> MSLGAKPFGEKKF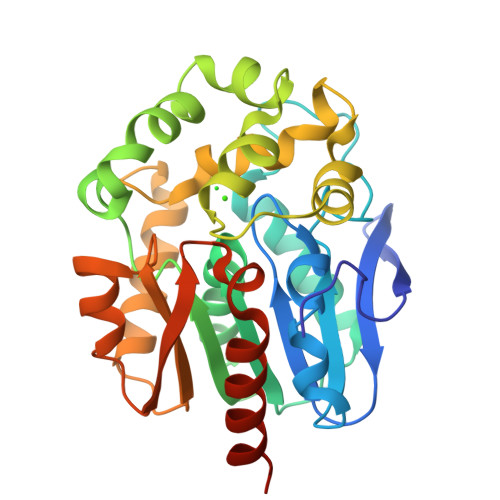IEIKGRRMAYIDEGTGDPILFQHGNPTSSYLWRNIMPHCAGLGRLIACDLIGMGDSDKLDPSGPERYTYAEHRDYLDALWEALDLGDRVVLVVHDWGSVLGFDWARRHRERVQGIAYMEAVAMPLEWADFPEQDRDLFQAFRSQAGEELVLQDNVFVEQVLPGLILRPLSEAEMAAYREPFLAAGEARRPTLSWPRQIPIAGTPADVVAIARDYAGWLSESPIPKLFINAEPGHLTTGRIRDFCRTWPNQTEITVAGAHFIQEDSPDEIGAAIAAFVRRLRPAHHHHHH>[2x]GPGSKPFSVPVLTVEEMTNSRFPIPLEKLFTGPSSAFVVQPQNGRCTTDGVL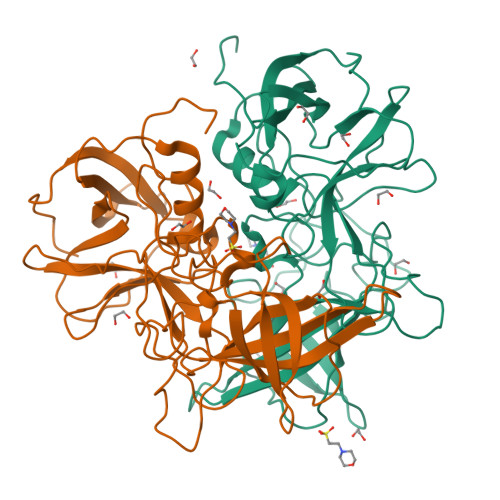LGTTQLSPVNICTFRGDVTHITGSRNYTMNLASQNWNNYDPTEEIPAPLGAPDFVGKIQGMLTQTTRADGSTRGHKATVYTGSADFAPKLGRVQFETDTDHDFEANQNTKFTPVGVIQDGSTTHRNEPQQWVLPSYSGRNTHNVHLAPAVAPTFPGEQLLFFRSTMPGCSGYPNMDLDCLLPQEWVQYFYQEAAPAQSDVALLRFVNPDTGRVLFECKLHKSGYVTVAHTGQHDLVIPPNGYFRFDSWVNQFYTLAPM>EETIPLQTLRCYNDYTSHITCRWADTQDAQRLVNVTLIRRVNEDLLEPVSCDLSDDMPWSACPHPRCVPRRCVIPCQSFVVTDVDYFSFQPDRPLGTRLTVTLTQHVQPPEPRDLQISTDQDHFLLTWSVALGSPQSHWLSPGDLEFEVVYKRLQDSWEDAAILLSNTSQATLGPEHLMPSSTYVARVRTRLAPGSRLSGRPSKWSPEVCWDSQPGDEAQPQNLECFFDGAAVLSCSWEVRKEVASSVSFGLFYKPSPDAGSAVLLREEECSPVLREGLGSLHTRHHCQIPVPDP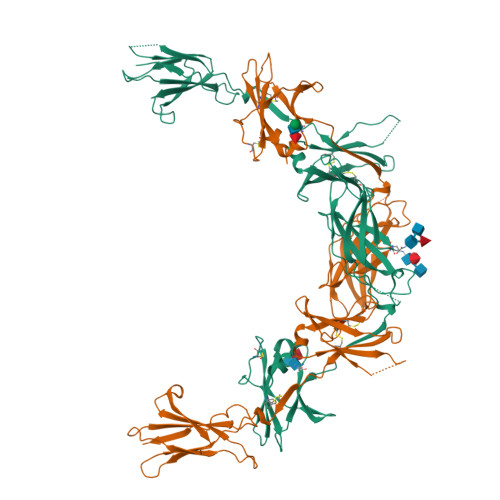ATHGQYIVSVQPRRAEKHIKSSVNIQMAPPSLQVTKDGDSYSLRWETMKMRYEHIDHTFEIQYRKDTATWKDSKTETLQNAHSMALPALEPSTRYWARVRVRTSRTGYNGIWSEWSEARSWDTE[2x]> DRFRSAVHREMIVAMTRTHLQNLLLKRFGTFKTQECRILASPAFSAVVLKAWASAVVDANLRLDGEGAMRLAYASPPPAVLSDPKVKE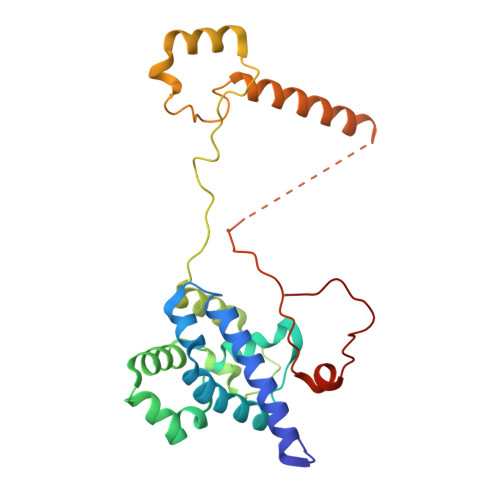LVASDPEAAWMLKKLSCQSVASFASLPREEEALEEVVRVKQKDNVPQPHFPSVLKMDHPQFPYEPHELEKMRDLYGVLLKWPYREQGQVASVAARRASLESKREERLRKGETEVAGQLKVTTGCSDSYVYAPSEMETGLYREHA> SAVLQ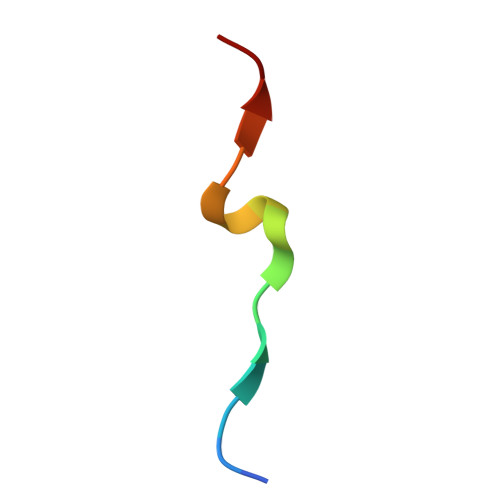KKITDYFHPKK>[12x]MRGKIYDRNGKVLAEDVERYKLVAVIDKKASANSKKPRHVVDKKETAKKLSTVINMKPEEIEKRLSQKKAFQIEFGRKGTNLTYQDKLKIEKMNLPGISLLPETERFYPNGNFASHLIGRAQKNPDTGELKGALGVEKIFDSYLSGSKGSLRYIHDIWGYIAPNTKKEKQPKRGDDVHLTIDSNIQVFVEEALDGMVERYQPKDLFAVVMDAKTGEILAYSQRPTFNPETGKDFGKKWANDLYQNTYEPGSTFKSYGLAAAIQEGAFDPDKKYKSGHRDIMGSRISDWNRVGWGEIPMSLGFTYSSNTLMMHLQDLVGADKMKSWYERFGFGKSTKGMFDGEAPGQIGWSNELQQKTSSFGQSTTVTPVQMLQAQSAFFNDGNMLKPWFVNSVENPVSKRQFYKGQKQIAGKPITK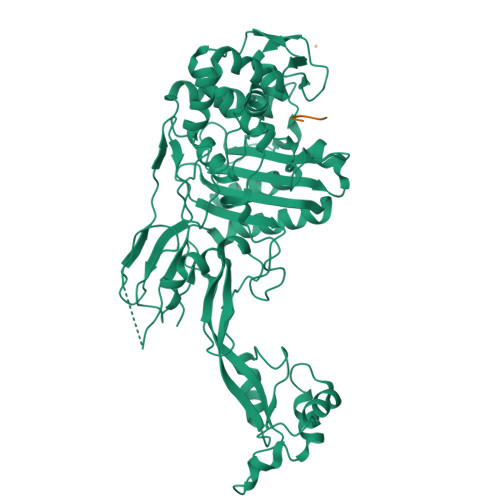DTAEKVEKQLDLVVNSKKSHAANYRIDGYEVEGKTGTAQVAAPNGGGYVKGPNPYFVSFMGDAPKKNPKVIVYAGMSLAQKNDQEAYELGVSKAFKPIMENTLKYLNVGKSKDDTSNAEYSKVPDVEGQDKQKAIDNVSAKSLEPVTIGSGTQIKAQSIKAGNKVLPHSKVLLLTDGDLTMPDMSGWTKEDVIAFENLTNIKVNLKGSGFVSHQSISKGQKLTEKDKIDVEFSS;>GGGGG[10x]>MGSSDEEEARELEERAREAAKRAIEAAKRTGDPRVRELAEELVKLAIWAAVEVWLDPSSSDVNEALKLIVEAIEAAVRALEAAERTGDPEVRELARELVRLAVEAAEEVQRNPSSSDVNEALKLIVIAIEAAVRALEAAERTGDPEVRELARELVRLAVEAAEEVQRNPSSEEVNEALRKIIKLILFAVMVLELAEEIGDPTWREMARR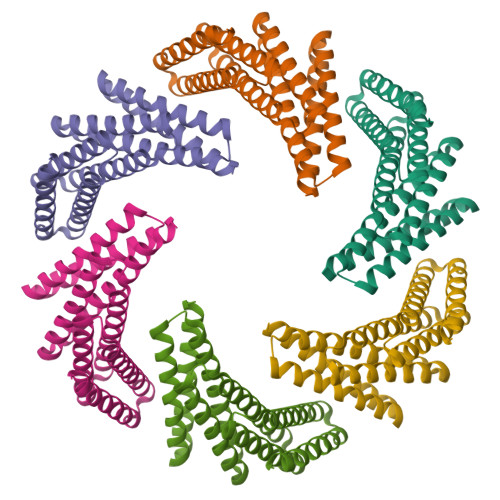AVREAVELAEEVQRDPSGWLGHGSLEHHHHHH[6x]>[2x]MSLLIRGATVVTHEESYRADVLCANGLIQAIGENLETPSGCDVLDGGGQYLMPGGIDPHTHMQLPFMGTVASEDFFSGTAAGLAGGTTSIIDFVIPN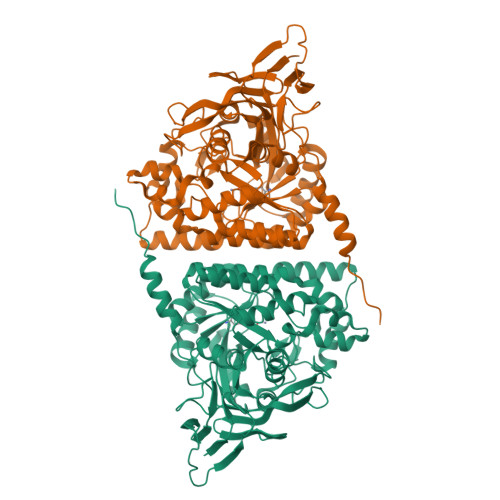PRQSLLEAFHTWRGWAQKSAADYGFHVAITWWSDEVAREMGELVAQHGVNSFKHFMAYKNAIMAADDTLVASFERCLELGAVPTVHAENGELVFHLQQKLLAQGLTGPEAHPLSRPPQVEGEAASRAIRIAETLGTPLYLVHISSREALDEIAYARAKGQPVYGEVLAGHLLLDDSVYRHPDWATAAGYVMSPPFRPVEHQEALWRGLQSGNLHTTATDHCCFCAEQKAMGRDDFSKIPNGTAGIEDRMALLWDAGVNSGRLSMHEFVALTSTNTAKIFNLFPRKGAIRVGADADLVLWDPQGSRTLSAATHHQRVDFNIFEGRTVRGIPSHTISQGKLLWAAGDLRAEPGAGRYVERPAYPSVYEVLGRRAERQRPVAVERHHHHHH>[4x]MSDLIEYSFYLTYAFLMTTGTITFIEALRTKNESVRHILNLETCISVVAAFFYSNFIGKLEHINYEEINLNRYVDWAITTPIMLLVLVLAFRVNQTNKAMVKFSDFMIILGMNYGMLGTGYLGDIGVIHKTMGTVLGFLFFGGLFYKLNTLRTSNASNDLLYGAFFVLWALYGVFYQMEQLPRNVGYNVLDLFSKCFVGIYFWAFYAKIFT;> MSDLIE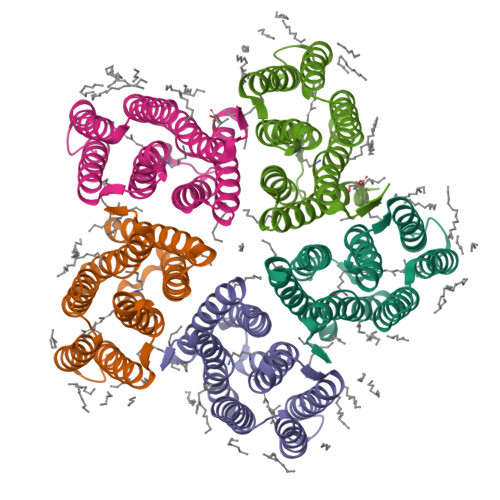YSFYLTYAFLMTTGTITFIEALRTKNESVRHILNLETCISVVAAFFYSNFIGKLEHINYEEINLNRYVDWAITTPIMLLVLVLAFRVNQTNKAMVKFSDFMIILGMNYGMLGTGYLGDIGVIHKTMGTVLGFLFFGGLFYKLNTLRTSNASNDLLYGAFFVLWALYGVFYQMEQLPRNVGYNVLDLFSKCFVGIYFWAFYAKIFTLEHHHHHH>[20x]GLAGRGVIYIPKDCQANRYLGTLNIRDMISDFKGVQYEKWITAGLVMPTFKIVIRLPANAFTGLTWVMSFDAYN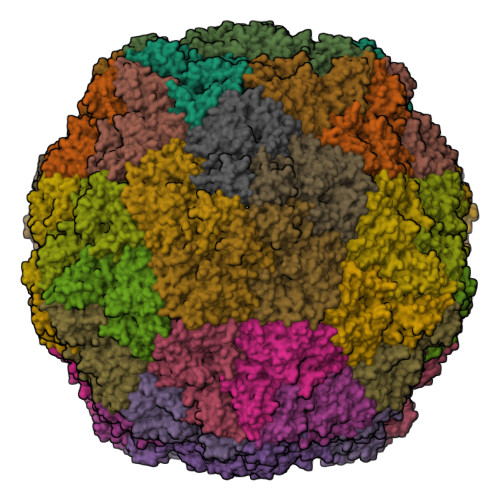RITSRITASADPVYTLSVPHWLIHHKLGTFSCEIDYGELCGHAMWFKSTTFESPRLHFTCLTGNNKELAADWQAVVELYAELEEATSFLGKPTLVFDPGVFNGKFQFLTCPPIFFDLTAVTALRSAGLTLGQVPMVGTTKVYNLNSTLVSCVLGMGGTVRGRVHICAPIFYSIVLWVVSEWNGTTMDWNELFKYPGVYVEEDGSFEVKIRSPYHRTPARLLADQSQRDMSSLNFYAIAGPIAPSGETAQLPIVVQIDEIVRPDLSLPSFEDDYFVWVDFSEFTLDKEEIEIGSRFFDFTSNTCRVSMGENPFAAMIACHGLHSGVLDLKLQWSLNTEFGKSSGSVTITKLVGDKAMGLDGPSHVFAIQKLEGTTELLVGNFAGANPNTRFSLYSRWMAIKLDQAKSIKVLRVLCKPRPGFSFYGRTSFPV> SMQQDIVNDHQEEAQGWKWEQIKEIIESGELARLKRSRQMTDKYHEHKKRTAGLDMNQYVLQKLGWSLDEPQLENAAAKAFSSSTLYAVRANDFPYNFEPGVVHLVLWSKVALPVHSPDKAVREAARARMNAFLQAQPLLRPLLSSGHVAWFVNYPELQSVARIFHAHVLLFFPRERYSAEQVKTTVDDILSHGFEPLA

We chose YPL067C, a yeast protein with no significant sequence similarity to any structure in the Protein Data Bank (PDB) as the target for our competition. In addition, YPL067C was chosen for its biological interest, as previous studies suggested that YPL067C is involved in preventing amyloid toxicity. Despite the lack of sequence homology to any protein in the PDB, a DALI16 search of YPL067C found that it is structurally similar to members of the widely conserved superfamily of histidine triad (HIT) proteins. YPL067C's characterization makes it the founding member of a new family we are calling HTC (for histidine triad with channel), with YPL067C being the first member, HTC1.

Crystals of this protein diffracted to 1.9 Å resolution. We asked all human competitors to build the best possible protein structure that they could given the protein sequence, a secondary structure prediction and an experimentally phased, density refined map of YPL067C. As a result, the top pruned Foldit structure was the overall highest-quality structure produced in the competition as measured by geometry, density fit and steric clashes. According to Molprobity, the top Foldit structure is an exceptional model, ranking in the 100th percentile in both its overall Molprobity score and clashscore of all structures in the PDB of similar resolution (1.95±0.25 Å). The superiority of the top Foldit structure can be attributed to better side-chain conformations than those in the top structure produced by the trained crystallographers. YPL067C's structure yielded unexpected insights into its biological function. Although YPL067C bears some resemblance to known HIT proteins, it is sequentially and structurally distinct. Its most notable distinguishing structural characteristic is an open channel not found in other HIT proteins. We find here that HTC1 is very effective in preventing in vitro amyloid formation of three model proteins, Aβ1–40, α-synuclein and reduced carboxy-methylated α-lactalbumin (RCMalA).>[2x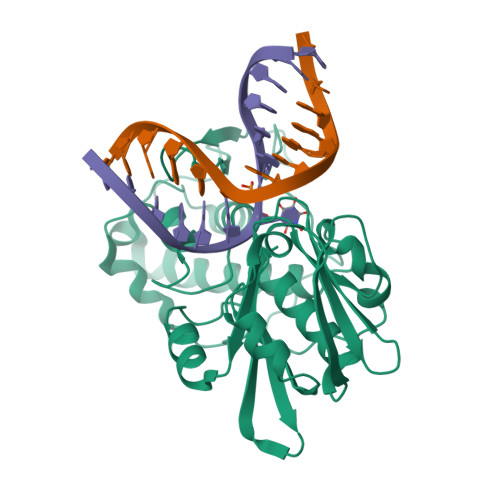]MPQGPEVALTADILEKYFKGKTLEYIDFISGRYSKSEPEGYDDFIANLPLKVSNVDTKGKFLWFELFDPNDKSNKWYIWNTFGLTGMWSLFEAKYTRAVLSFDNELMAYFSDMRNFGTFKFSNSEKELKRKLNELGPDFLKNDDIDISKIKKYKQPIVALLMDQKKIGSGLGNYLVAEILYRAKIDPHKLGSNLTDQEIENLWYWIKYETKLAYDSNHIGYMVNLENESSKIGRKNYHPNIHPTEKEFDFLVYRKKKDPNGNKVIADKIIGSGKNKRTTYWAPAIQKLEHHHHHH> RTITGDTCNEETQNLSTIYLREYQSKVK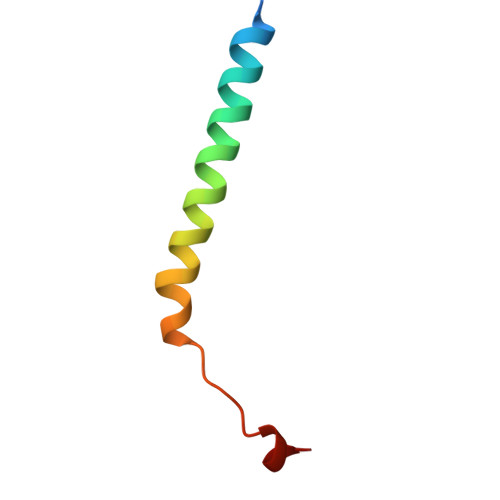RQIFSDYQSEVDIYNRI4-[3-[3-[2,6-bis(azanyl)-5-(3-chlorophenyl)pyrimidin-4-yl]propoxy]phenoxy]butanoic acid | C23 H25 Cl N4 O4 | 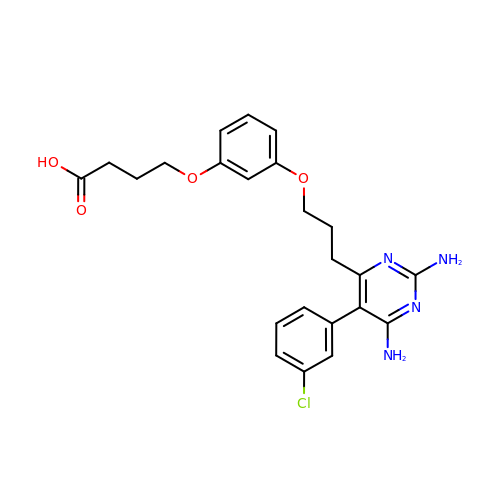OXGBDAHIBSSGDL-UHFFFAOYSA-N The psychrophilic aromatic aminotransferase from Psychrobacter sp. B6 is a representative of pyridoxal phosphate (PLP)-dependent enzymes. PsyArAT exhibits an activity typical for ArAT: transamination, which is a transfer of an amine group between aromatic α-amino acids and α-ketoacids. The mechanism of active site adjustment toward substrates of psychrophilic aromatic amino acid aminotransferase (PsyArAT) from Psychrobacter sp. B6 is discussed based on crystal structures of complexes with four hydroxy-analogs of substrates: phenylalanine, tyrosine, tryptophan and aspartic acid. These competitive inhibitors are bound in the active center of PsyArAT but do not undergo transamination reaction, which makes them an outstanding tool for examination of the enzyme catalytic center.

In the case of PsyArAT/FOH and PsyArAT/YOH, the ASU is created by a functional dimer; in PsyArAT/DOH the asymmetric unit represented only a monomer, but the functional dimer is reproduced with the symmetry-related molecule. Despite the presence of an inhibitor in the pockets of chain B of PsyArAT/YOH and PsyArAT/FOH dimers, the non-bound form of PLP was present, similarly, as it was in the catalytic center at both monomers of the native enzyme structure. In the PsyArAT/FOH complex, the closest distance between the ligand and PLP (measured from the α-hydroxyl group of the inhibitor to aldehyde carbon of PLP) was 4.1 Å in monomer A and 3.3 Å in monomer B, while in the PsyArAT/YOH structure respective distances were bigger (5.7 Å and 4.6 Å). In the catalytic center of both complexes, the Arg280* switch was in the “down” position; however, in the case of PsyArAT/YOH, it was placed a little deeper than in the PsyArAT/FOH complex. In the subunit A, Arg280*, which was pushed down by a YOH ligand, made two hydrogen bonds between guanidine moiety nitrogen atoms and carboxyl oxygens of Asp11 (2.8 Å and 3.5 Å). In monomer B, only one contact was present with Asp11 (2.9 Å), but another bond was created with the hydroxyl group of Asn132 (3.5 Å). Despite the similar size and aromatic character of FOH and YOH ligands, motions in the structure of PsyArAT complexed with the phenylalanine analog were slightly more significant. The kink on the long helix H14 was at least two times bigger for PsyArAT/FOH (~6° in monomer A and ~4.5° in monomer B) than for PsyArAT/YOH (~1.5° in monomer A and ~2.0° in monomer B). Movements of the N-terminal (~2.7 Å/A, ~3.0 Å/B) and C-terminal (~2.2 Å/A, 1.7 Å/B) parts of the small domain were also bigger for the PsyArAT/FOH complex than for PsyArAT/YOH (~1.2 Å/A, 1.8 Å/B and ~0.5 Å/A, ~1.0 Å/B, respectively). Interestingly, the volume of the pockets in one monomer was much smaller than in the second one of the dimer in all complexes (excluding PsyArAT/DOH), but the difference in the case of FOH bound caused a smaller disparity between them than in the case of YOH present in the active center.

>[2x]MFERIDYYAGDPILGLVEKFAADNNPDKVNLGIGIYYDESGVMPVLDCVKIAEQRIADPISPRPYLPMAGLPGHRKGCQELLFGKDAPVLKDGLVATIATIGGSGALKVGAEFIHEWFPQSKCYVSDPTWGNHIAIFEGCDIEVGKYPYYDTATGGIKFDEMIAFFETLNKDDVLLLHPCCHNPTGVDLTREQWDTVLNVIQERELIPFMDIAYQGFGEDMDSDAYAIRKAVDMGLPLFVSNSFSKNLSLYGERVGGLSVVCPTVDETERVFGQLNSTVRRIYSSPPSHGGRVVDIVMNDAALHEQWVGEVYAMRDRIKSMRTKLKSVLEAKISGRNFDYLTAQNGMFSFTGLTPEQVERLQSEFGIYMISNSRMCVAGLNSSNIDYVANAMVDVLKD> GMPQTAIGRQLVESGMANDVTLDNESVVRDGIKLNELAFKTFGESQHIFVATIDLNELTFTPATKDDKNVPATGPESSAPLPIHAFAAEANGKTVWLGVNGDYYADNPRRVMGLFYKDGVCINSQYFEGHDEVLYQLKNGETYVGQADEA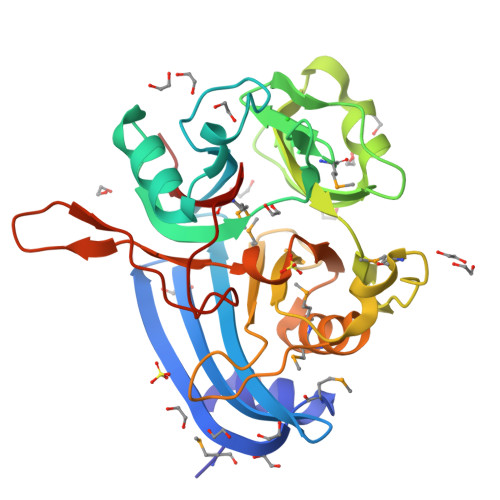LAHEANLLHALGGYGLLVKDGVVQNFYEEMGDLQNTHPRTSVGLSQDRKTMYVFVVDGRRKDSFFALGLTLPHLATMMKAVGCYNAINLDGGGSTTLIIRKVNDGGKPTFPILNTPADDRVPRKVTNSMLIIEKK>GPGDYKDDDDKDAPQLLHFVDQYREQLIARVTSVEVVLDKLHGQVLSQEQYERVLAENTRPSQMRKLFSLSQSWDRKCKDGLYQALKE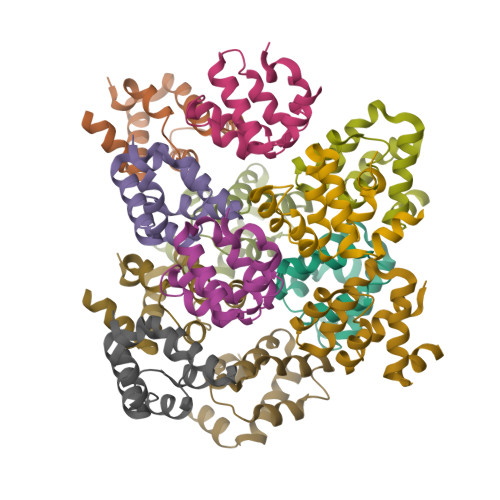THPHLIMELWEKGSKK[12x]> VPDEWEVAREKITMSRELGQGSFGMVYEGVAKGVVKDEPETRVAIKTVNEAASMRERIEFLNEASVMKEFNCHHVVRLLGVVSQGQPTLVIMELMTRGDLKSYLRSLRPEMENNPVLAPPSLSKMIQMAGEIADGMAYLNANKFVHRDLAARNCMVAEDFTVKIGDFGMTRDIYETDYYRKGGKGLLPVRWMSPESLKDGVFTTYSDVWSFGVVLWE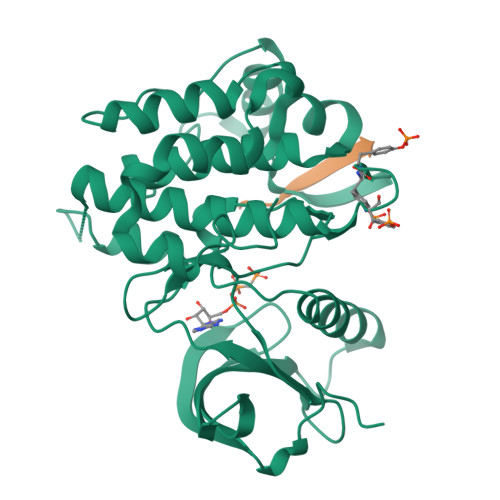IATLAEQPYQGLSNEQVLRFVMEGGLLDKPDNCPDMLLELMRMCWQYNPKMRPSFLEIISSIKEEMEPGFREVSFYYSEENK;> KKKSPGEYVNIEFG> SNAMPYTWKFLGISKQLSLENGIAKLNQLLNLEVDLDIQTIRVPSDPDGGTAADEYIRYEMRLDISNLDEGTYSKFIFLGNSKMEVPMFLCYCGTDNRNEVVLQWLKAEYGVIMWPIKFEQKTMIKLADASIVHVTKENIEQITWFSSKLYFEPETQDKNLRQFSIEIPRESCEGLALGYGNTMHPYNDAIVPYIYNETGMAVERLPLTSV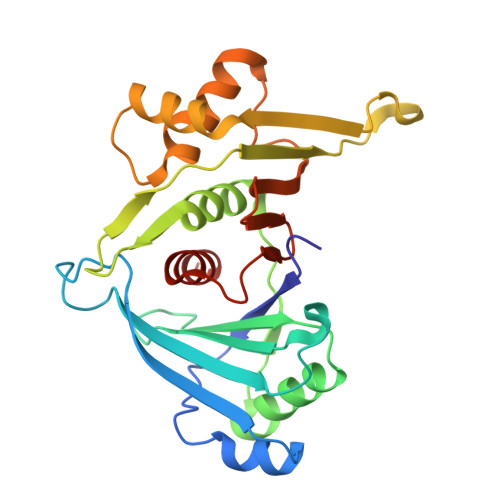ILAGHTKIMRESIVTSTRSLRNRVLAVVLQSIQF>APADNAADARPVDVSVSIFINKIYGVNTLEQTYKVDGYIVAQWTGKPRKTPGDKPLIVENTQIERWINNGLWVPALEFINVVGSPDTGNKRLMLFPDGRVIYNARFLGSFSND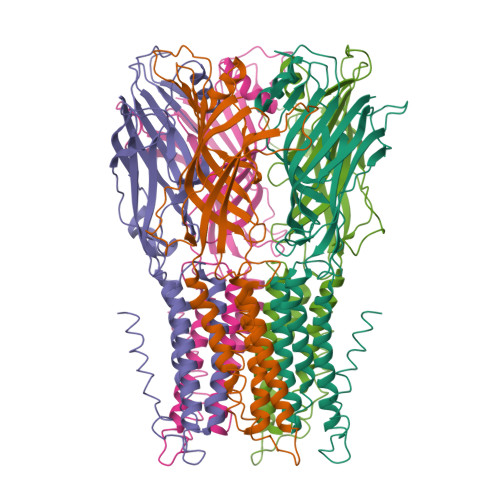MDFRLFPFDRQQFVLELEPFSYNNQQLRFSDIQVYTENIDNEEIDEWWIRKASTHISDIRYDHLSSVQPNQNEFSRITVRIDAVRNPSYYLWSFILPLGLIIAASWSVFWLESFSERLQTSFTLMLTVVAYAFYTSNILPRLPYTTVIDQMIIAGYGSIFAAILLIIFAHHRQANGVEDDLLIQRCRLAFPLGFLAIGCVLVIRGITL[10x]> MTGMSREEVESLIQEVLEVYPEKARKDRNKHLAVNDPAVTQSKKCIISNKKSQPGLMTIRGCAYAGSKGVVWGPIKDMIHISHGPVGCGQYSRAGRRNYYIGTTGVNAFVTMNFTSDFQEKDIVFGGDKKLAKLIDEVETLFPLNKGISVQSECPIGLIGDDIESVSKVKGAELSKTIVPVRCEGFRGVSQSLGHHIANDAVRDWVLGKRDEDTTFASTPYDVAIIGDYNIGGDAWSSRILLEEMGLRCVAQWSGDGSISEIELTP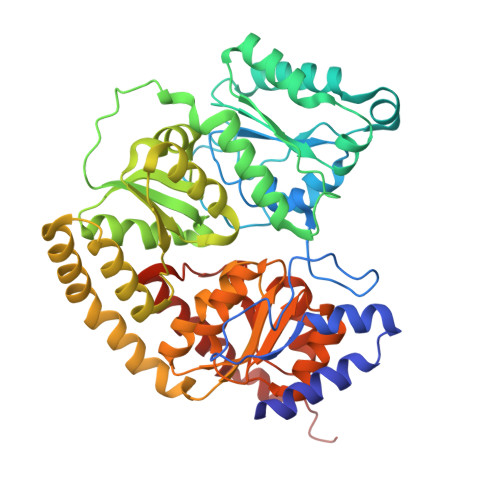KVKLNLVHCYRSMNYISRHMEEKYGIPWMEYNFFGPTKTIESLRAIAAKFDESIQKKCEEVIAKYKPEWEAVVAKYRPRLEGKRVMLYIGGLRPRHVIGAYEDLGMEVVGTGYEFAHNDDYDRTMKEMGDSTLLYDDVTGYEFEEFVKRIKPDLIGSGIKEKFIFQKMGIPFREMHSWDYSGPYHGFDGFAIFARDMDMTLNNPCWKKLQAPWE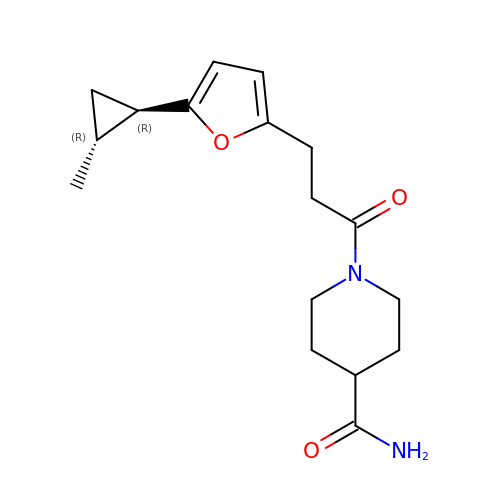1-[3-[5-[(1~{R},2~{R})-2-methylcyclopropyl]furan-2-yl]propanoyl]piperidine-4-carboxamide | C17 H24 N2 O3 | KDDWUCROKBAIBA-BXUZGUMPSA-N> TEFKAGSAKKGATLFKTRCLQCHTVEK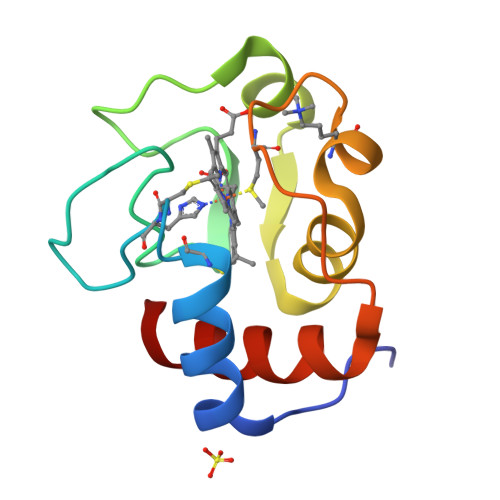GGPHKVGPNLHGIFGRHSGQAEGYSYTDAIIKKNVLWDENNMSEYLTNPKKYIPGTKMAFGGLKKEKDRNDLITYLKKACE>MKGPAFEFAVAMMKRNASTVKTEYGEFTMLGIYDRWAVLPRHAKPGPTILMNDQEVDVVDAKELVDKDGTNLELTLLKLNRNEKFRDIRGFLTREEAEVNEAVLAINTSKFPNMYIPVGQVTDYGFLNLGGTPTKRMLMYNFPTRAGQCGGVLMSTGKVLGIHVGGN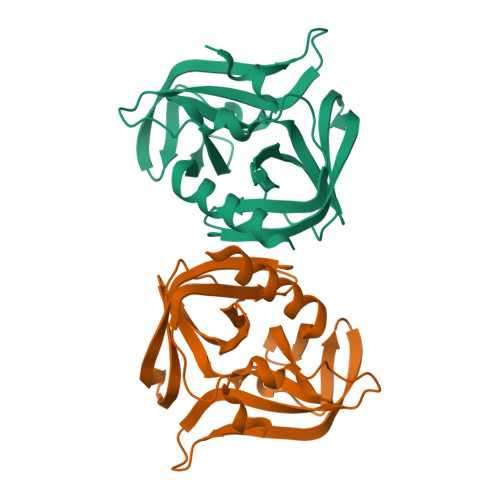GHQGFSAALLRHYFND[2x]>MSIPFTRWPEEFARRYREKGYWQDLPLTDILTRHAASDSIAVIDGERQLSYRELNQAADNLACSLRRQGIKPGETALVQLGNVAEL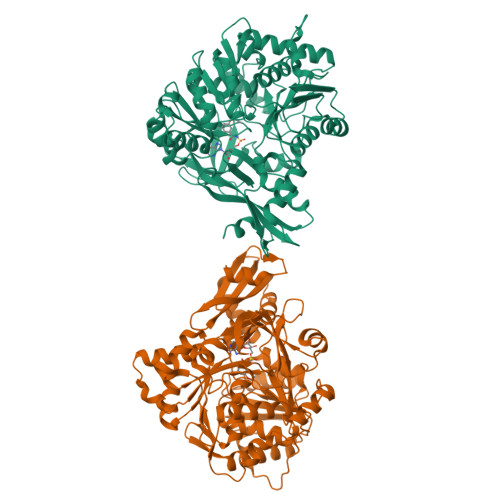YITFFALLKLGVAPVLALFSHQRSELNAYASQIEPALLIADRQHALFSGDDFLNTFVTEHSSIRVVQLLNDSGEHNLQDAINHPAEDFTATPSPADEVAYFQLSGGTTGTPKLIPRTHNDYYYSVRRSVEICQFTQQTRYLCAIPAAHGYAMSSPGSLGVFLAGGTVVLAADPSATLCFPLIEKHQVNVTALVPPAVSLWLQALIEGESRAQLASLKLLQVGGARLSATLAARIPAEIGCQLQQVFGMAEGLVNYTRLDDSAEKIIHTQGYPMCPDDEVWVADAEGNPLPQGEVGRLMTRGPYTFRGYYKSPQHNASAFDANGFYCSGDLISIDPEGYITVQGREKDQINRGGEKIAAEEIENLLLRHPAVIYAALVSMEDELMGEKSCAYLVVKEPLRAVQVRRFLREQGIAEFKLPDRVECVDSLPLTAVGKVDKKQLRQWLASRASATNSSSVDKLAAALEHHHHHH[2x]> MSNLSKGTGSRKDTKMRIRAFPMTMDEKYVNSIWDLLKNAIQEIQRKNNSGLSFEELYRNAYTMVLHKHGEKLYTGLREVVTEHLINKVREDVLNSLNNNFLQTLNQAWNDHQTAMVMIRDILMYMDRVYVQQNNVENVYNLGLIIFRDQVVRYGCIRDHLRQTLLDMIARERKGEVVDRGAIRNACQMLMILGLEGRSVYEEDFEAPFLEMSAEFFQMESQKFLAENSASVYIKKVEARINEEIERVMHCLDKSTEEPIVKVVERELISKHMKTIVEMENSGLVHMLKNGKTEDLGCMYKLFSRVPNG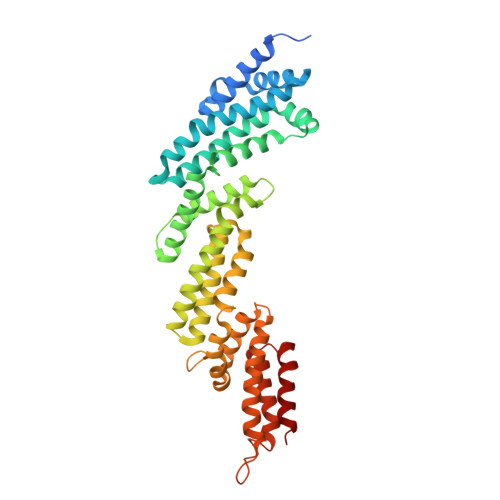LKTMCECMSSYLREQGKALVSEEGEGKNPVDYIQGLLDLKSRFDRFLLESFNNDRLFKQTIAGDFEYFLNLN>[4x]SNAMDNEKGLLIVLSGPSGVGKGTVRKRIFEDPSTSYKYSISMTTRQMREGEVDGVDYFFK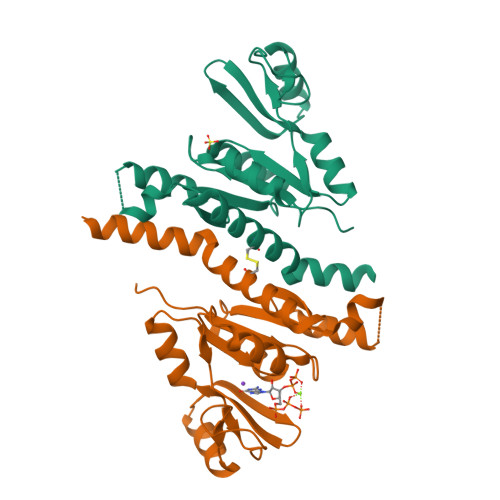TRDAFEALIKDDQFIEYAEYVGNYYGTPVQYVKDTMDEGHDVFLEIEVEGAKQVRKKFPDALFIFLAPPSLEHLRERLVGRGTESDEKIQSRINEARKEVEMMNLYDYVVVNDEVELAKNRIQCIVEAEHLKRERVEAKYRKMILEAKK>MIGEGDDIGSSNNLEKQSHGLRISDRDHFQRLREECRSDPGEFHGRLAKREICWLIEGPGGNPAWAFYDDAAETWTGWDASSAAPITLDLPESFEPWERAFNDDDPPNWRWFEGGLTSTAFNEVDRHVLSGHGDEAAMIFEGDRWNMASEGGRGGPVDSEVISRRKLLLESAKCALALKALGLEAGDRIALNMPSIPEQIYWTEGAKRMGIVYTPVFGGFSDKTLSDRIADAGARVVVTADGSYRNAQMVPFKPSYTDPALDNFIAVPVAMELLGQALEDGELVVAPEHAGLIRSEVAGLLDGEVTVERSDVMRGVGKALTAIASGEAAGGAMTPRQAAQLRIAIASALVDSPPRVDAVVVVKHTAQPDLPWNEARDHWSHDLTAAAGEELLKAARDAGFDVADEEALLALSDTEFVRAIWAGAPVLAVDAEYPNFIIYTSGSTGKPKGVVHVHGGYASGVAATMPAAFGAEPGDVMYVVADPGWITGQSYQIAASLLSRVTTVITEGSPVFPHAGRFASIIERYGVNVFKAGVTFLKSVMQNPENLKDIQRYDLSSLKVATFCAEPVSPAVQAFAMEHITHRYINSYWATEHGGMVWTHFADADGFPLEADAHTYPLPWIMGDVWVEDADGSSNGPVEYERDTGTGGAPWRVAEDGEKGEIVIALPYPYLTRTIWGDVENFTVEHVGNLARVAGGWRGDEVRYADTYWRRWKGAWAYTQGDFAMRHPDGSFSLHGRSDDVINVSGHRIGTEEIEGAILRDKALDPNSPVGNVIVIGAPHSQKGVTPIAFVTPVEGRRLTQDDKRRLTDLVRTEKGAVAVPQDFIELSEFPETRSGKYMRRMVRAVVEGGEVGDASTLRNPESLDELARAVDGWKRRQSLSDTQALFERYRFFTIQYNLVAPGKRVATVTVKNPPVNALNERALDELVIIAEHLARKDDVAAVVFTGSGTASFVAGADIRQMLEEVNSVEEAKALPDNAQLAFRTIEEMDKPCIAAIQGVALGGGMEFALACHYRVAEPKARFGQPEINLRLLPGYGGTQRLPRLLADGGGETGLRDALDLILGGRAIDADAALAVGAVDALADGSDNALSHAHAMVREFVRSGDDSALGKAFAARKTQTQSWHEPASIDLDAVLEDEFLQRILNQLEWAGRDKAGERALDAVRTGWTQGMTAGLECEAQRFAEAIIDPEGGKTGIQQFMDKQSPPLPVRRDGVWEDDQHEATKTALIEAGDLLPLGAPFYPGVTAIPPKQLAFGIARDPDTGAPRFGPPETHERELVVNTPKPGANEALIYLLSSEVNFNDIWALTGIPVSPFDAHDEDVQITGSGGLALVAALGSELKEEGRLQVGDLVSVYSGTSELLSPLAGDDPMYAGFAIQGYETKTGSHAQFLTVQGPQLHRPPADLTLEQAGAYTLNLGTVARCLFTTLEIQAGKTAFVEGSATGTGLDALKSSVRTGLAVTGLVSSEDRAEFVKSHGSVGAINRKDPEIADCFTPVPDDPDEARQWEADGEKLLDAYRETNGGKLADYVVSHAGERAFPRSFQLLAEGGRLAFYGASSGYHFSFMGKGGEARPDEMLARANLRGGESVLLYYGPGSHELADEKGLEMVEAA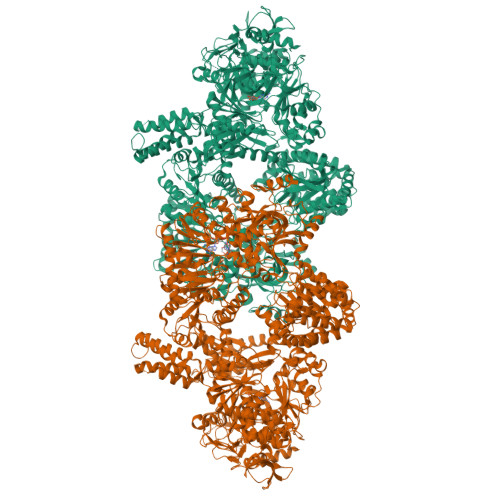RLMKARMVIVTTSDGQREFLQSLGLEDAVEGIVSIEGLKRRLSDFHWPDTLPRLPDARTDIENFKIGVRAYQQNTMKPFGTAVGKLLRSPGNPRGVPDLVIERAGQDTLGVSTSLVKPFGGRVIYAEEMAGRRYTFYAPQVWTRQRRIYMPSAEIFGTHLCNAYEVTMMNEMVAAGLLDVTEPTMVPWEGLPEAHQAMWDNRHSGATYVVNHALPAMGLTTKDELLEYWVAAQSDTGETS[2x]>[4x]MKTISFNFNQFHQNEEQLKLQRDARISSNSVLELTKVVNGVPTWNSTGRALYAKPVQVWD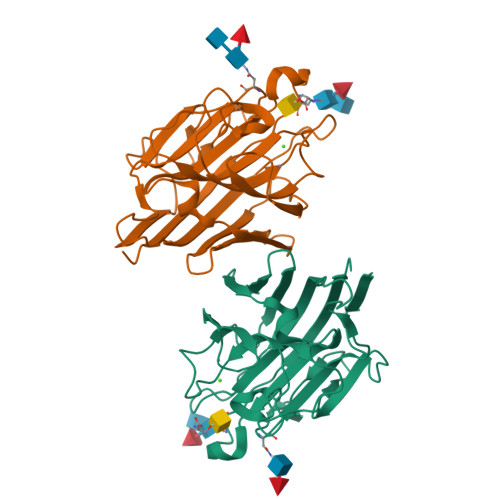STTGNVASFETRFSFSIRQPFPRPHPADGLVFFIAPPNTQTGEGGGYFGIYNPLSPYPFVAVEFDTFRNTWDPQIPHIGIDVNSVISTKTVPFTLDNGGIANVVIKYDASTKILHVVLVFPSLGTIYTIADIVDLKQVLPESVNVGFSAATGDPSGKQRNATETHDILSWSFSASLPGTNEF>MEKVPGEMEIERRERSEELSEAERKAVQAMWARLYANSEDVGVAILVRFFVNFPSAKQYFSQFKHMEDPLEMERSPQLRKHASRVMGALNTVVENLHDPDKVSSVLALVGKAHALKHKVEPVYFKILSGVILEVVAEEFA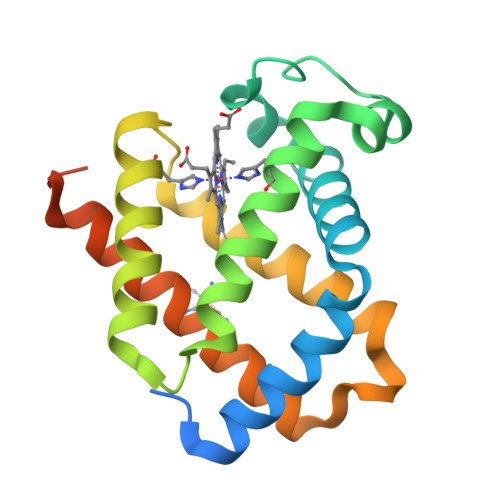SDFPPETQRAWAKLRGLIYSHVTAAYKEVGWVQQVPNATTPPATLPSSGP[2x]> ANPEQLKHCNGILKELLSKKHAAYAWPFYKPVDASALGLHDYHDIIKHPMDLSTVKRKMENRDYRDAQEFAADVRLMFSNCYKYNPPDHDVVAMARKLQDVFEFRYAKMPD

The BET family proteins (BRD2, BRD3, BRD4, and BRDT) contain two tandem bromodomains and an extra-terminal domain at the C-terminal. The BET family proteins generally recognize acetylated histones H3 and H4 (and references therein); however, BRD2 preferentially recognize mono/di-acetylated histone tail of H4. The tertiary structure of all bromodomains contains a left-handed α-helical bundle formed by four α-helices (αZ, αA, αB, and αC). The α-helical bundle along with flanking ZA and BC loops create a deep hydrophobic cavity, which recognizes a specific sequence of acetylated-histone tails.

In both our apo- and the BD2-L10 complex crystal structures, the side chains of several residues are observed to display multiple conformations. Three of the conserved water molecules both in our apo-BD2 and in the BD2-L10 complex, are displaying alternate positions. In apo-BD2, the alternate positions of water molecules are reciprocated by the alternate conformations of some of the surrounding residues (N424, C425). The dynamic nature of these water molecules, as demonstrated by alternate positions, might have a possible role in facilitating the binding of Kac into the binding pocket. The binding pocket apo-BD2 residues, displaying a different conformation compared to H4K5ac complex, are mostly in the BC loop region (C425, H433, and D434). Compared to the H4K5ac complex, the C425 side chain is flipped, both in our apo- and BD2-L10 structures. In the apo-form, C425 contributes an extra water mediated hydrogen bond to N429-NH2. This water molecule is unique to our apo- structure, and it is not observed in the previously reported structures. Alternate position of conserved active site water molecules along with this newly observed water molecule, demonstrate a flexible hydration shell in the binding pocket. Overall, these structural variations together demonstrate a dynamic nature of the binding site, necessary for the activity of the BD2.> MADLYPTGQQISFQTTPLNVQDPTRMMNLDQSSPVARNETQNGGGIAHAEFAMFNSKRLESDLEAMGNKIKQHEDNLKFLKSQKNKMDEAIVDLQVHMSK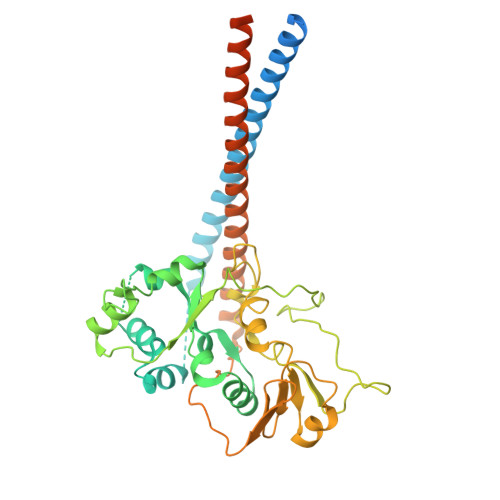LNSSPTPRSENSDNSLQGEDINAQILRHENSAAGVLSLVETLHGAQASQLMLTKGVVGVVAKLGKVNDENLSQILSNYLGTRSMLAVVCRNYESVTALEAYDNHGNIDINAGLHCLGSSIGREIGDSFDAICLENLRPYVGQHIADDLQRRLDLLKPKLPNGECPPGFLGFAVNMIQIDPAYLLCVTSYGYGLRETLFYNLFSRLQVYKTRADMISALPCISDGAVSLDGGIIRKTGIFNLGNRDEVNVRFAKPTASRTMDNYSEAEKKMKELKWKKEKTLEDIKREQVLREHAVFNFGKKKEEFVRCLAQSSCTNQPMNTPRGTLESGKETAAAKFERQHMDSSTSAA> MTTVTATVHDISGRPDDSHWTFSSDLREQDGVIITPRVVRVKPFNGELALTLPPGPVRVTHHQDRWLIDVPEEDSDLWDLIE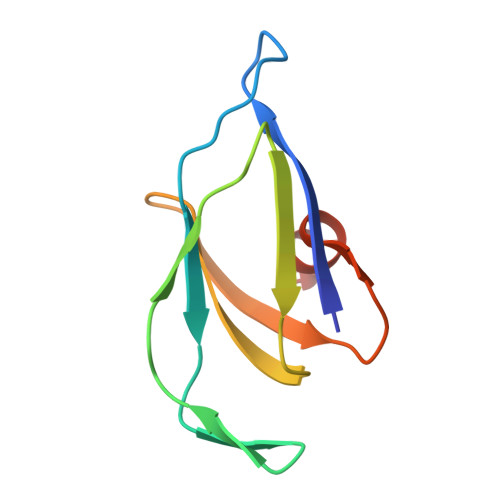AATD N-[(1S)-2-{[(3S)-1-benzyl-3-cyanopyrrolidin-3-yl]amino}-1-(cyclohexylmethyl)-2-oxoethyl]morpholine-4-carboxamide 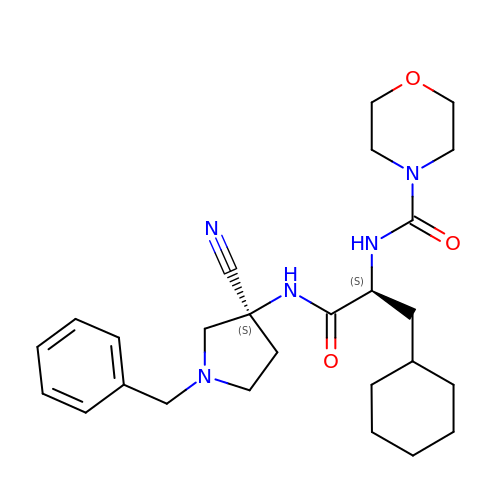| C26 H37 N5 O3 | OHVQFYYBGNOGJV-JYFHCDHNSA-N2-{[(3alpha,5alpha,7alpha,8alpha,10alpha,12alpha,17alpha)-3,12-bis{2-[(4-O-alpha-D-glucopyranosyl-beta-D-glucopyranosyl)oxy]ethoxy}cholan-7-yl]oxy}ethyl 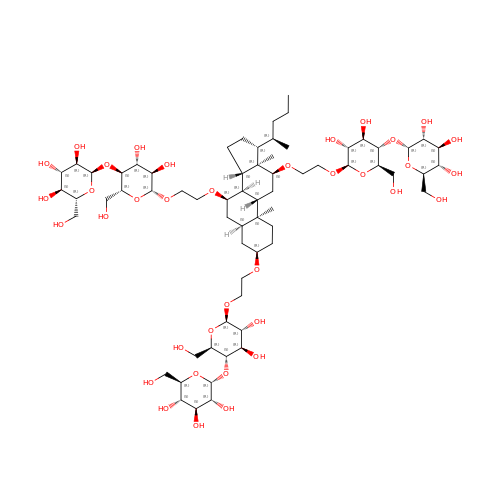4-O-alpha-D-glucopyranosyl-beta-D-glucopyranoside | C66 H114 O36 | YGUVIEOMNBFSRV-GLUVFYGUSA-N In the present work, we report the kinetic and structural characterization of the isoenzyme GSTM1-1 from Camelus dromedarius (CdGSTM1-1). Upon entering the living cell, xenobiotic and toxic compounds may undergo GST-mediated conjugation with glutathione (GSH) in order to become more soluble and to be excreted by the cell. Two domains are recognized in each monomer: the conserved N-terminal thioredoxin-like domain, containing the GSH binding site (G-site), and the less conserved C-terminal domain, containing the xenobiotic binding site (H-site). Kinetics analysis showed that the enzyme displays a relative narrow substrate specificity and restricted ability to bind xenobiotic compounds.

The crystal structures of CdGSΤM1-1 were determined by X-ray crystallography in complex with the substrate (GSH) or the reaction product (S-p-nitrobenzyl-GSH), providing snapshots of the induced-fit catalytic mechanism. The crystal structure of CdGSTM1-1 in complex with GSH or S-(p-nitrobenzyl)-GSH was resolved by X-ray crystallography at 2.55 and 2.05 Å resolution, respectively. Pro39 (CdGSTM1-1 numbering) appears to be highly conserved in mu class GSTs and is responsible for providing a characteristic extended loop connecting β2 and α2 from domain I. The ligands, S-(p-nitrobenzyl) glutathione (GTB), bound to the G-site (GSH part) and H-site (nitro-benzyl moiety) of CdGSTM1-1, and formic acid (FMT), bound to the H-site, are shown in Figure 7A. Notably, a move of loop β2-α2 upon binding of S-p-nitrobenzyl-GSH (~4 Å) was observed, which may suggest an induced-fit mechanism to facilitate the binding of various substrates. Similarly, Trp8 and Leu13 are found to be conserved in all compared structures and are involved in the stabilization of GTB moiety in the active site via H-bonding interaction and pi-alkyl interaction with the nitro-benzyl ring, respectively. The carbonyl oxygen of Gln72 and carboxyl group of Asp106 are likely to form an H-bond with the γ-Glu amino moiety of GTB. The amide group and side chain hydroxyl group of Ser73 are found to be H-bonded to the α-carboxyl group of GTB. Arg43 and Lys50 are located 3.09 Å and 3.52 Å, respectively, from the carboxylate glycine end of GTB, and are involved in the formation of a salt bridge with GTB contributing to the stability of GTB in the active site. The bound xenobiotics compound, formic acid (FMT), is found to interact via weak van der Waals forces with the GTB moiety in the G-site. The more compact and well-packaged structure upon S-p-nitrobenzyl-GSH binding, as a consequence of the ~4 Å movement of the loop β2-α2, may contribute favorably to the overall structural stability of the S-hexyl-GSH complex, compared to the free and the GSH-bound enzyme.

>[4x]MPMILGYWDIRGLAHAIRLLLEYTGSDYEEKIYSMGDAPDYDRSQWLSEKFKLGLDFPNLPYLIDGAHRLTQSNAILRYIARKHNLCGETEEEKIRVDVLENQAMDTRLDFARVCYNPDFEKLKPGFLKEIPEKMKLFSEFLGKRTWFAGDKLNYVDFLAYDVLDVYRIFEPKCLDEFPNLKDFMSRFEGLKKISAYMKSSRFLRSPLFLKMAMWGNK COPI mediates retrograde trafficking from the Golgi to the endoplasmic reticulum (ER) and within the Golgi stack, sorting transmembrane proteins bearing C-terminal KKxx or KxKxx motifs. The heptameric COPI complex (α/β/β'/γ/δ/ε/ζ) is recruited en bloc onto Golgi membranes (Hara-Kuge et al., 1994) but can be divided conceptually into two subcomplexes. The α/β'/ε B-subcomplex has been likened to clathrin because α-COP, β'-COP, and clathrin contain N-terminal WD-repeat (also referred to as β-propeller) domains and C-terminal α-solenoid domains and because recent studies have suggested that β'-COP, like clathrin, can form trimers. We demonstrate that N-terminal WD-repeat domains of α- and β'-COP directly bind dilysine motifs and establish the molecular bases for the interactions using X-ray crystallography, structure-directed mutagenesis, and isothermal titration calorimetry (ITC).

In contrast, we do not observe trimer formation of the N-terminal WD-repeat domain in any of our structures of either β'1-304 with different peptides (Supplemental Experimental Procedures) or β'1-604 with CTFKTKTN. One explanation for the poor fit is the significant conformational flexibility within β'-COP as indicated by comparing our structure of β'1-604 with CTFKTKTN with the unliganded structure. Flexibility in the COPI coat is in line with cryo-EM reconstructions and cryoelectron tomography data (Faini et al., 2012). It may be that once the N-terminal WD-repeat domains are anchored to the membrane by cargo binding, flexibility between the two WD-repeat domains of β'-COP, and likely also α-COP, may facilitate assembly of polymeric coats having a range of geometries with local but no global point group symmetry. Flexibility between β'-COP WD-repeat domains and the location of cargo binding have implications for COPI coat assembly.

> MKLDIKKTFSNRSDRVKGIDFHPTEPWVLTTLYSGRVELWNYETQVEVRSIQVTETPVRAGKFIARKNWIIVGSDDFRIRVFNYNTGEKVVDFEAHPDYIRSIAVHPTKPYVLSGSDDLTVKLWNWENNWALEQTFEGHEHFVMCVAFNPKDPSTFASGCLDRTVKVWSLGQSTPNFTLTTGQERGVNYVDYYPLPDKPYMITASDDLTIKIWDYQTKSCVATLEGHMSNVSFAVFHPTLPIIISGSEDGTLKIWNSSTYKVEKTLNVGLERSWCIATHPTGRKNYIASGFDNGFTVLSLGNDEPTLSLDPVGKLVWSGGKNAAASDIFTAVIRGNEEVEQDEPLSLQTKELGSVDVFPQSLAHSPNGRFVTVVGDGEYVIYTALAWRNKAFGKCQDFVWGPDSNSYALIDETGQIKYYKNFKEVTSWSVPMHSAIDRLFSGALLGVKSDGFVYFFDWDNGTLVRRIDVNAKDVIWSDNGELVMIVNTNSNGDEASGYTLLFNKDAYLEAANNGNIDDSEGVDEAFDVLYELSESITSGKWVGDVFIFTTATNRLNYFVGGKTYNLAHYTKEMYLLGYLARDNKVYLADREVHVYGYEISLEVL;> CTFKTKTN>VKMAETCPIFYDVFFAVANGNELLLDLSLTKVNATEPERTAMKKIQDCYVENGLISRVLDGLVMTTISSSKDCMGEAVQNTVEDLKLNTLGREICPAVKRDVDLFLTGTPDEYVEQVAQYKALPVVLENARILKNCVDAKMTEEDKENALSLLDK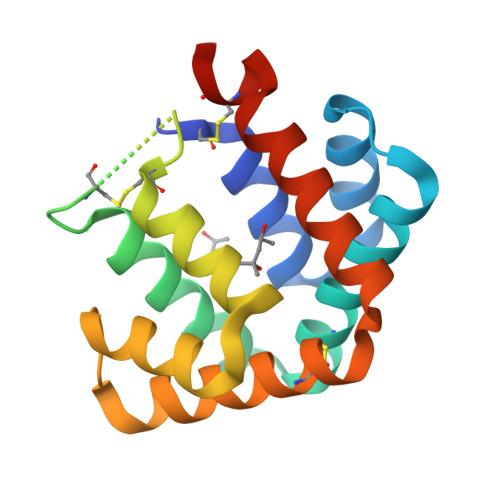IYTSPLCLEHHHHHH[2x]>[3x]SLGTTTAPARTLVNQSPNLKIEFEISRESNSVIRIKSFFTNLSSSPISN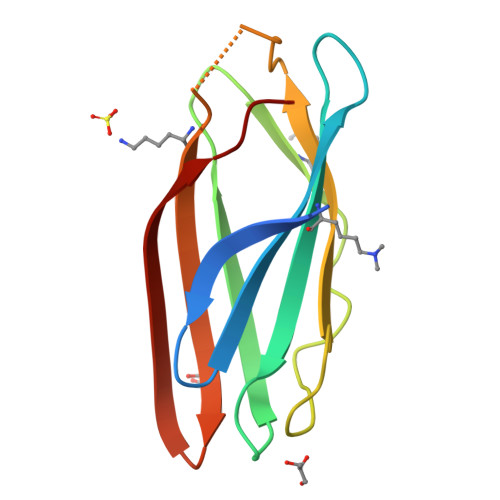LVFLLAVPKSMSLKLQPQSSNFMIGNAKDGISQEGTIENAPANPSKALKVKWKVNYSVNSTQAEETAVFTLPNV METHACRYLYL-COENZYME A | C25 H40 N7 O17 P3 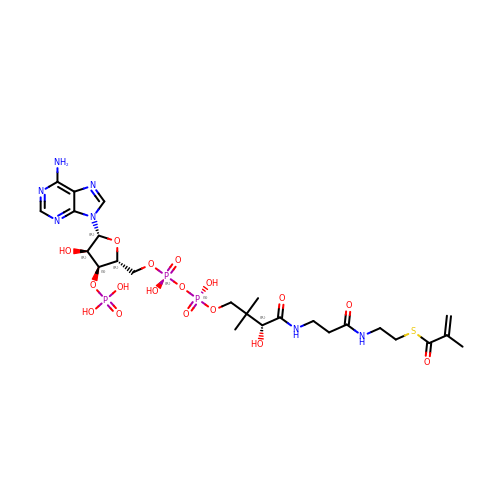S | NPALUEYCDZWBOV-NDZSKPAWSA-N> AEMRIGHGFDVHAFGGEGPIIIGGVRIPYEKGLLAHSDGDVALHALTDALLGAAALGDIGKLFPDTDPAFKGADSRELLREAWRRIQAKGYTLG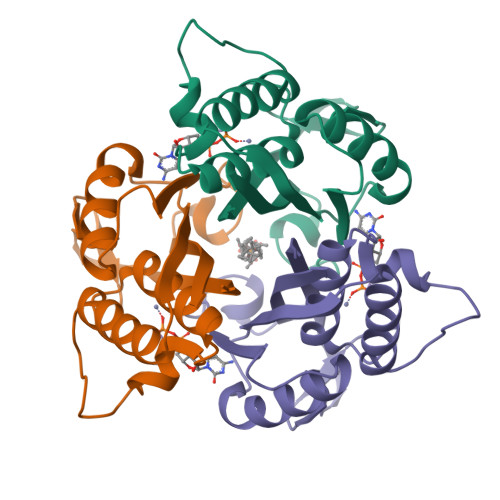NVDVTIIAQAPKMLPHIPQMRVFIAEDLGCHMDDVNVKATTTEKLGFTGMGLGIACEAVALLIKATK>[3x]MALKNNTLWTGPKPEANCIIEYGKQNPDSKLTLILVKNGGIV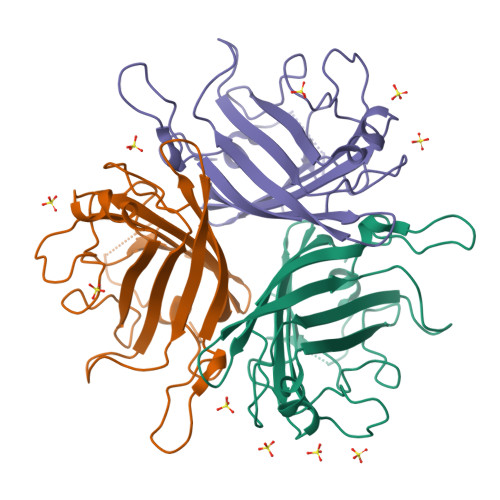NGYVTLMGASDYVNTLFKNKNVSINVELYFDATGHILPDSSSLKTDLELKYKQTADFSARGFMPSTTAYPFDLPNAGTHNENYIFGQCYYKASDGALFPLEVTVMLNKRLPDSRTSYVMTFLWSLNAGLAPETTQATLITSPFTFSYIREDD> MPSFNPVRFLELPIDIRKEVYFHLDGNFCGAHPYPIDILYKSNDVELPGKPSYKRSKRSKKLLRYMYPVFATYLNIFEYSPQLIEKWLEYAFWLRYDCLVLDCFKVNHLYDGTLIDALEWTYLDNELRLAYFNKASMLEVWYTFKEYKKWVIDSVAFDELDLLNVSNIQFNIDNLTPQLVDKCLSILEQKDLFATIGEVQFGQDEEVGEEKDVDVSGANSDENSSPSSTIKNKKRSASKRSHSDNGNVGATHNQLTSISVIRTIRSMESMKSLRKITVRGEKLYELLINFHGFRDNPGKTISYIVKRRINEIRLSRMNQISRTGLADFTRWDNLQKLVLSRVAYIDLNSIVFPKNFKSLTMKRVSKIKWWNIEENILKELKVDKRTFKSLYIKEDDSKFTKFFNLRHTRIKELDKSEINQITYLRCQAIVWLSFRTLNHIKLQNVSEVFNNIIVPRALFDSKRVEIYRCEKISQVLVI;> MFNRTTQLKSKHPCSVCTRRKVKCDRMIPCGNCRKRGQDSECMKSTKLITASSSKEYLPDLLLFWQNYEYWITNIGLYKTKQRDLTRTPANLDTDTEECMFWMNYLQKDQSFQLMNFAMENLGALYFGSIGDISELYLRVEQYWDRRADKNHSVDGKYWDALIWSVFTMCIYYMPVEKLAEIFSVYPLHEYLGSNKRLNWEDGMQLVMCQNFARCSLFQLKQCDFMAHPDIRLVQAYLILATTTFPYDEPLLANSLLTQCIHTFKNFHVDDFRPLLNDDPVESIAKVTLGRIFYRLCGCDYLQSGPRKPIALHTEVSSLLQHAAYLQDLPNVDVYREENSTEVLYWKIISLDRDLDQYLNKSSKPPLKTLDAIRRELDIFQYKVDSLEEDFRSNNSRFQKFIALFQISTVSWKLFKMYLIYYDTADSLLKVIHYSKVIISLIVNNFHAKSEFFNRHPMVMQTITRVVSFISFYQIFVESAAVKQLLVDLTELTANLPTIFGSKLDKLVYLTERLSKLKLLWDKVQLLDSGDSFYHPVFKILQNDIKIIELKNDEMFSLIKGLGSLVPLNKLRQESLLEEEDENNTEPSDFRTIVEEFQSEYNISDILS;> MFNRITASSSKEYLPDLLLFWQNYEYWITNIGLYKTKQRDLTRTPANLDTDTEECMFWMNYLQKDQSFQLMNFAMENLGALYFGSIGDISELYLRVEQYWDRRADKNHSVDGKYWDALIWSVFTMCIYYMPVEKLAEIFSVYPLHEYLGSNKRLNWEDGMQLVMCQNFARCSLFQLKQCDFMAHPDIRLVQAYLILATTTFPYDEPLLANSLLTQCIHTFKNFHVDDFRPLLNDDPVESIAKVTLGRIFYRLCGCDYLQSGPRKPIALHTEVSSLLQHAAYLQDLPNVDVYREENSTEV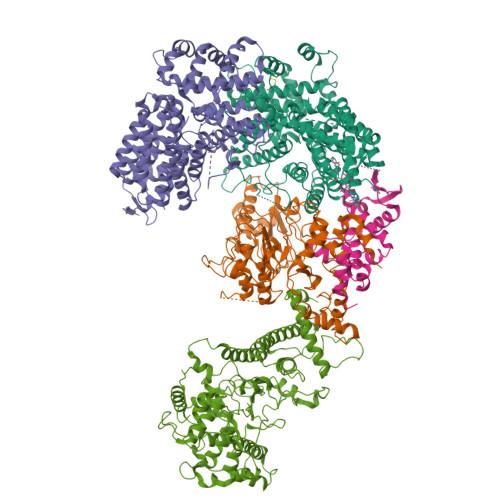LYWKIISLDRDLDQYLNKSSKPPLKTLDAIRRELDIFQYKVDSLEEDFRSNNSRFQKFIALFQISTVSWKLFKMYLIYYDTADSLLKVIHYSKVIISLIVNNFHAKSEFFNRHPMVMQTITRVVSFISFYQIFVESAAVKQLLVDLTELTANLPTIFGSKLDKLVYLTERLSKLKLLWDKVQLLDSGDSFYHPVFKILQNDIKIIELKNDEMFSLIKGLGSLVPLNKLRQESLLEEEDENNTEPSDFRTIVEEFQSEYNISDILS;> MVTSNVVLVSGEGERFTVDKKIAERSLLLKNYLNDMHDSNLQNNSDSESDSDSETNHKSKDNNNGDDDDEDDDEIVMPVPNVRSSVLQKVIEWAEHHRDSNFPDEDDDDSRKSAPVDSWDREFLKVDQEMLYEIILAANYLNIKPLLDAGCKVVAEMIRGRSPEEIRRTFNIVNDFTPEEEAAIRRENEWAEDR;> MRSSILFLLKLMKIMDVQQQQEAMSSEDRFQELVDSLKPRTAHQYKTYYTKYIQWCQLNQIIPTPEDNSVNSVPYKDLPISAELIHWFLLDTLITDDKPGEKREETEDLDEEEENSFKIATLKKIIGSLNFLSKLCKVHENPNANIDTKYLESVTKLHTHWIDSQKAITTNETNNTNTQVLCPPLLKVSLNLWNPETNHLSEKFFKTCSEKLRFLVDFQLRSYLNLSFEERSKIRFGSLKLGKRDRDAIIYHKVTHSAEKKDTPGHHQLLALLPQDCPFICPQTTLAAYLYLRFYGIPSVSKGDGFPNLNADENGSLLQDIPILRGKSLTTYPREETFSNYYTTVFRYCHLPYKRREYFNKCNLVYPTWDEDTFRTFFNEENHGNWLEQPEAFAFPDKIPFDFKKIMNFKSPYTSYSTNAKKDPFPPPKDLLVQIFPEIDEYKRHDYEGLSQNSRDFLDLMEVLRERFLSNLPWIYKFFPNHDIFQDPIFGNSDFQSYFNDKTIHSKGSPILSFDILPGFNKIYKNKTNFYSLLIERPSQLTFASSHNPDTHPTQKQESEGPLQMSQLDTTQLNELLKQQSFEYVQFQTLSNFQILLSVFNKIFEKLEMKKSSRGYILHQLNLFKITLDERIKKSKIDDADKFIRDNQPIKKEENIVNEDGPNTSRRTKRPKQIRLLSIADSSDESSTEDSNVFKKDGESIEDGAYGENEDENDSEMQEQLKSMINELINSKISTFLRDQMDQFELKINALLDKILEEKVTRIIEQKLGSHTGKFSTLKRPQLYMTEEHNVGFDMEVPKKLRTSGKYAETVKDNDDHQAMSTTASPSPEQDQEAKSYTDEQEFMLDKSIDSIEGIILEWFTPNAKYANQCVHSMNKSGNKSWRANCEALYKERKSIVEFYIYLVNHESLDRYKAVDICEKLRDQNEGSFSRLAKFLRKWRHDHQNSFDGLLVYLSN> MFTSKSGGAIGPFHSVAEAAGCVKTTDWMFLTLLFLAVLGGYHIHFMLTAGDWDFWVDWKDRRMWPTVVPILGVTFAAAAQAFFWENFKLPFGATFAVSGLLIGEWINRYCNFWGWTYFPISLVFPSALVVPALWLDIIMLLSGSYVITAVVGSLGWGLLFYPNNWPAIAALHQATEQHGQLMSLADLVG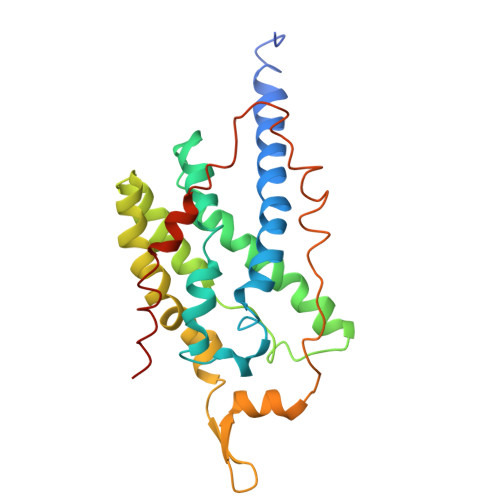FHFVRTSMPEYIRMVERGTLRTFGKEVVPVAAFFSGFVSMMVYFLWWFVGKWYSTTKVIQKI>MAEKIPKPVSKRLVSYYMCLERLLDEGVEVVSSEELARRLDLKASQIRKDLSYFGEFGKRGVGYNVEHLYDAIGEILGVKKEWKLVVVGAGNIGRAVANYTVMKEKGFRIIGIFDSDPSKIGKEAAPGLTVSDVSE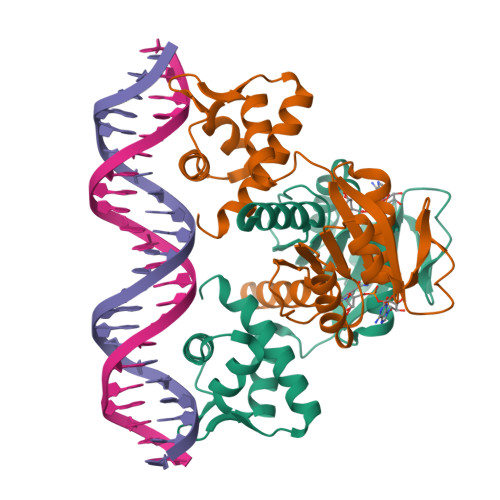LEKFVEEHGVEIGVIAVPAEHAQEIAERLEKAGIKGILNFAPVKIKVSVPVENIDITASLRVLTFEIVRRNS[2x]> PDESSADVVFKKP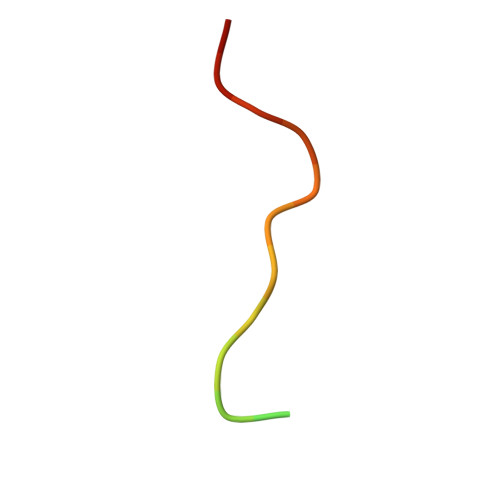LAPAPR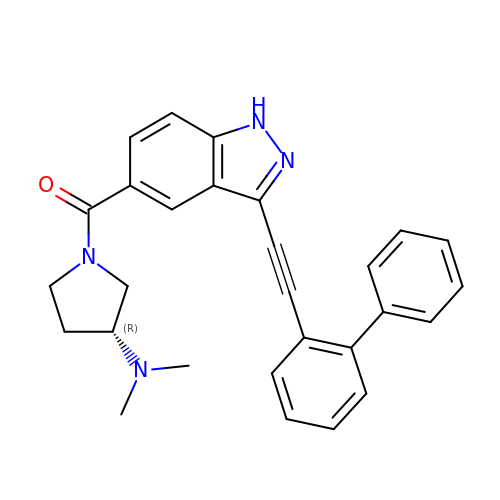{3-[([1,1'-biphenyl]-2-yl)ethynyl]-1H-indazol-5-yl}[(3R)-3-(dimethylamino)pyrrolidin-1-yl]methanone | C28 H26 N4 O | ZRBBUAGMFWALNG-HSZRJFAPSA-N CYTIDINE-3'-MONOPHOSPHATE 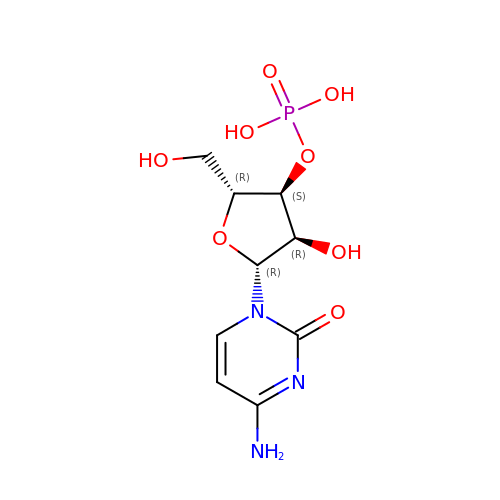| C9 H14 N3 O8 P | UOOOPKANIPLQPU-XVFCMESISA-N(2Z)-9-oxodec-2-enoic acid | C10 H16 O3 | 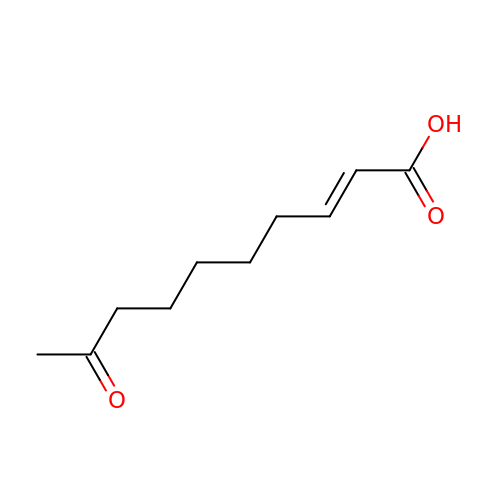INJRDZMWIAYEMM-VURMDHGXSA-N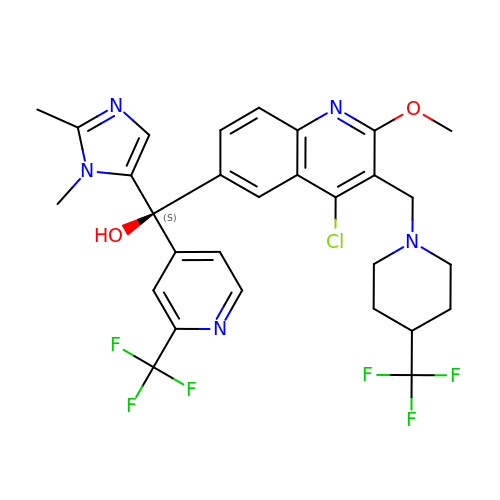(S)-(4-chloro-2-methoxy-3-{[4-(trifluoromethyl)piperidin-1-yl]methyl}quinolin-6-yl)(1,2-dimethyl-1H-imidazol-5-yl)[2-(trifluoromethyl)pyridin-4-yl]methanol | C29 H28 Cl F6 N5 O2 | SXCAASBRTBWENF-MHZLTWQESA-N6,7-dimethoxy-2,4-dihydro-1~{H}-isoquinolin-3-one | C11 H13 N O3 | 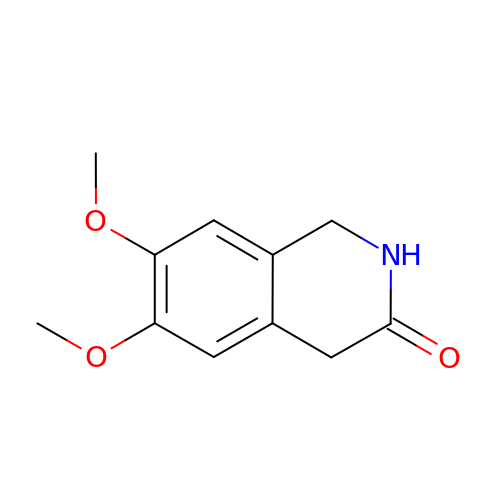FRBTVJSVXIIDIG-UHFFFAOYSA-N>YFGKLESKLSVIRNLNDQVLFIDQGNRPLFEDMTDSDCRDNAPRTIFIISMYKDSQRRGMAVTISVACAAASTLSCENKIISFKEMNPPDNIKDTKSDIIFFQRRVPGHDNKMQFESSSYEGYFLACEKE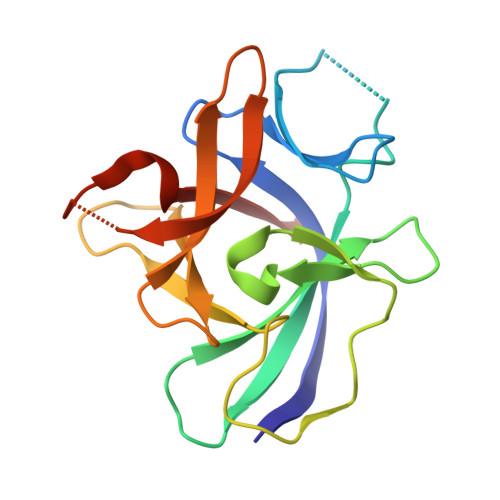RDLFKLILKKEDELGDRSIMFTVQNED[2x]> TQVFDLEGYGAISRAMGGTSSSYYTGNAALISNPATLSFAPDGNQFELGLDVVTTDIKVHDSHGAEPKSSTYAVGAQLSYVAQLDDWRFGAGLFVSSLGTEYGSKSFLSQTENGIQTSFDNSSRLIVLRAPIGFSYQATSKLTFGASVDLVWTSLNLELLLPSSQVGALTAQGNLSGGLVPSLAGFVGTGGAAHFSLSRNSTAGGAVDAVGWGGRLGLTYKLTDNTVLGAMYNFKTSVGDLEGKATLSAISGDGAVLPLDGDIRVKNFEMPASLTLGLAHQFNERWVVAADIKR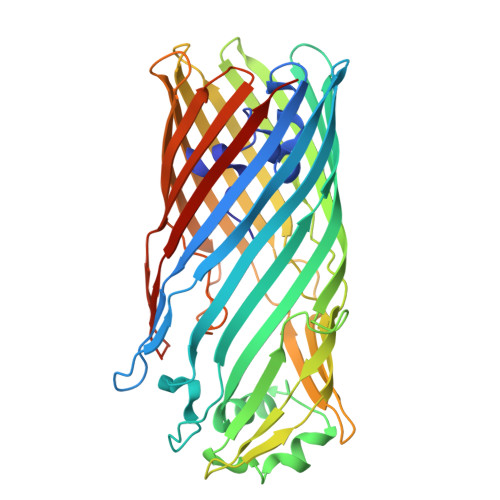AYWGDVMDSMNVAFISQLGGIDVALPHRYQDITVASIGTAYKYNNDLTLRAGYSYAQQALDSELILPVIPAYLKRHVTFGGEYDFDKDSRINLAISFGLRERVQTPSYLAGTEMLRQSHSQINAVVSYSKNFHHHHHH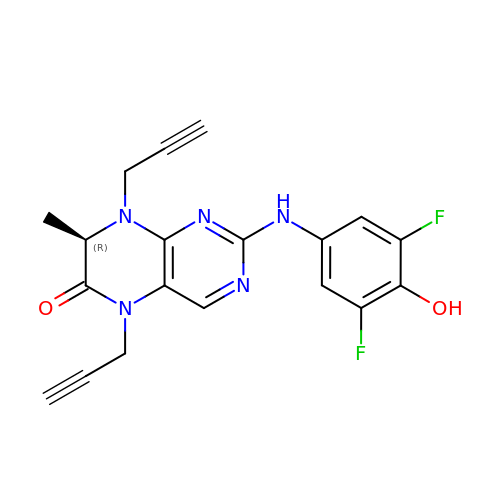(7R)-2-[(3,5-difluoro-4-hydroxyphenyl)amino]-7-methyl-5,8-di(prop-2-yn-1-yl)-7,8-dihydropteridin-6(5H)-one | C19 H15 F2 N5 O2 | KDZIESJUFYBJGD-LLVKDONJSA-N>AKDPSWASILQGLEEPYHTFVERLNVALDNGLPEGTPKDPILRSLAYSNANKECQKLLQARGHTNSPLGDMLRACQAWTPKDKTKVL[6x]

Human T-cell Leukaemia Virus type 1 (HTLV-1) is an untreatable retrovirus that causes lethal malignancies and degenerative inflammatory conditions. Here, we show that high-resolution crystal structures of the mature-length HTLV-1c CA protein define essential lattice interfaces and identify a distinct ligand-binding pocket. Across the known Orthoretrovirinae, CA is a two-domain protein with HIV being the best characterised. However, our structures reveal that HTLV-1 does still have a pocket formed between helices 3, 4, and 5, albeit an electropositive one capable of binding to either phosphate or sulfate in vitro.

To obtain higher resolution, we expressed residues A128-L214 (CACTD), which were purified as a dimer and crystallised in space group P212121 with diffraction to 1.47 Å resolution. The structure revealed a short 310 helix followed by α-helices 8 to 11. The asymmetric unit comprised 6 copies with two possible dimer configurations: one mediated by helix 9, and the other by an interdigitation of residues R188 and H190 in the 10-11 loop. Comparison to the HIV-1 CA CTD dimer crystal structure suggested the former as the biologically relevant dimer interface, but this was not unambiguous due to structural differences in this region. To improve the CA full-length structure, we re-solved it by molecular replacement searching for three independent copies of the refined CACTD structure as a search model. This unbiased approach returned a CTD dimer virtually identical to that mediated by α-helix 9 in the CACTD structure (RMSD = 1.580 Å), suggesting that this is the biologically relevant dimer interface. Curiously, while this residue is well-resolved in the electron density map from the CACTD structure, it makes an aromatic stacking interaction with its counterpart in the dimer partner that necessitates a breaking of the two-fold symmetry. The positive dihedral value observed for our CTD dimer supports the presence of the immature arrangement in our crystal packing. Y113F was chosen in order to remove only the hydroxyl group of the side chain, which binds to a water molecule, bridging this residue to the sulfate/phosphate groups. Lastly, while we were confident in our assignment of the biologically-relevant CACTD dimer interface, we decided to test mutants at both this interface (Y174A), and the alternative interface suggested by the interdigitation observed in the CACTD crystal packing (R188A, and H190A – see Supplementary Fig. 3g). Unsurprisingly, Y174A reduced infectivity to zero, albeit without affecting particle production.>[4x]TTIVSVRRNGHVVIAGDGQATLGNTVMKGNVKKVRRLYNDKVIAGFAGGTADAFTLFELFERKLEMHQGHLVKAAVELAKDWRTDRMLRKLEALLAVADETASLIITGNGDVVQPENDLIAIGSGGPYAQAAARALLENTELSAREIAEKALDIAGDICIYTNHFHTIEELSYK;>HHHHHHSEMTPREIVSELDKHIIGQDNAKRSVAIALRNRWRRMQLNEELRHEVTPKNILMIGPTGVGKTEIARRLAKLANAPFIKVEATKFTEVGYVGKEVDSIIRDLTDAAVKMVRVQAIEKNRYRAEELAEERILDVLIPPAKNNWGQTEQQQEPSAARQAFRKKLREGQLDDKEIEIDLAAAPMGVEIMAPPGMEEMTSQLQSMFQN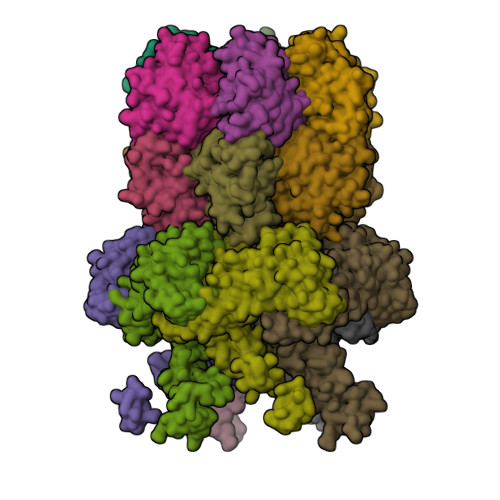LGGQKQKARKLKIKDAMKLLIEEEAAKLVNPEELKQDAIDAVEQHGIVFIDQIDKICKRGESSGPDVSREGVQRDLLPLVEGCTVSTKHGMVKTDHILFIASGAFQIAKPSDLIPELQGRLPIRVELQALTTSDFERILTEPNASITVQYKALMATEGVNIEFTDSGIKRIAEAAWQVNESTENIGARRLHTVLERLMEEISYDASDLSGQNITIDADYVSKHLDALVADEDLSRFIL[2x]>MAHHHHHHTDLKASSLRALKLMDLTTLNDDDTDEKVIALCHQAKTPVGNTAAIVIYPRFIPIARKTLKEQGTPEIRIATVTNFPHGNDDIDIALAETRAAIAYGADEVDVVFPYRALMAGNEQVGFDLVKACKEACAAANVLLKVIIETGELKDEALIRKASEISIKAGADFIKTSTGKVAVNAT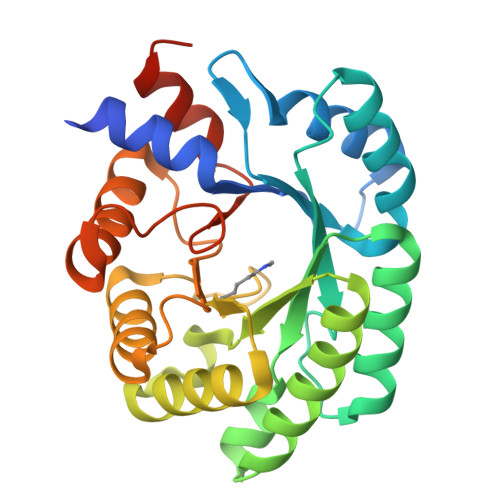PESARIMMEVIRDMGVEKTVGFKPAAGVRTAEDAQKYLAIADELFGADWADARHYRFGASDLLASLLKALGHGDGKSASSY[2x]>[2x]SLMADEIAKAQVARPGGDTIFGKIIRKEIPAKIIFEDDRCLAFHDISPQAPTHFLVIPKKHISQ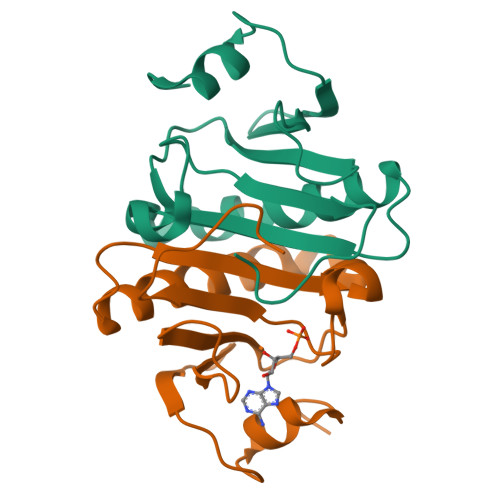ISVAEDDDESLLGHLMIVGKKCAADLGLNKGYRMVVNEGSDGGQSVYHVHLHVLGGRQMHWPPG> GAMADTCMSRIVKEYKVILKTLASDDPIANPYRGIIESLNPIDETDLS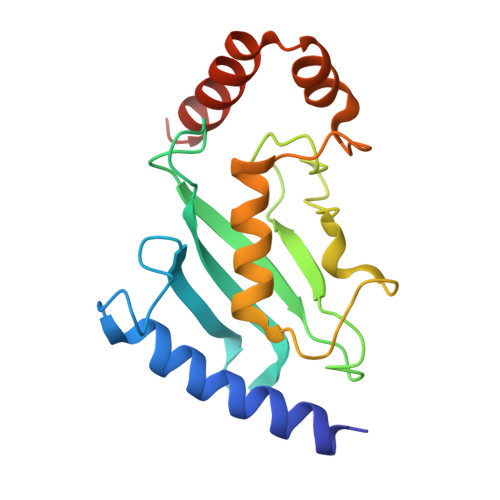KWEAIISGPSDTPYENHQFRILIEVPSSYPMNPPKISFMQNNILHSNVKSATGEICLNILKPEEWTPVWDLLHCVHAVWRLLREPVSDSPLDVDIGNIIRCGDMSAYQGIVKYFLAERERINNH>GPYASLTEIEHLVQSVCKSYRETCQ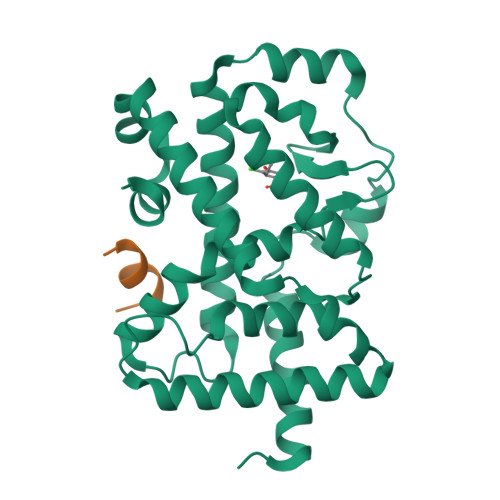LRLEDLLRQRSNIFSREEVTGYQRKSMWEMWERCAHHLTEAIQYVVEFAKRLSGFMELCQNDQIVLLKAGAMEVVLVRMCRAYNADNRTVFFEGKYGGMELFRALGCSELISSIFDFSHSLSALHFSEDEIALYTALVLINAHRPGLQEKRKVEQLQYNLELAFHHHLSKTHRQSILAKLPPKGKLRSLCSQHVERLQIFQHLHPIVVQAAFPPLYKELFSTETESPVGLSK[2x];>[2x]NSHQKVTLLQLLLGHKNEEN> MRGSHHHHHHGSV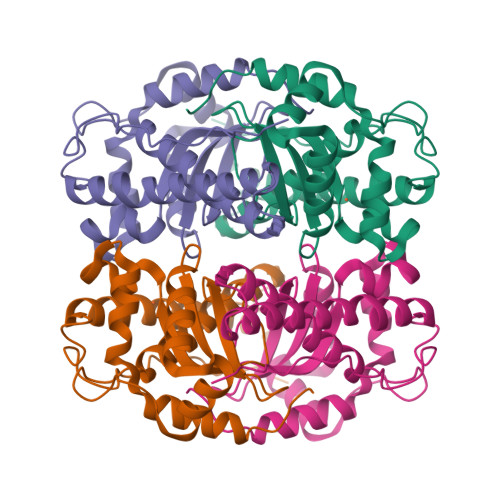VSLKRYELPPLPYNYDALEPIISAETLRYHHDKHHLGYVNGANAALDKLEKYLNGQLTDIDVRAVSRDFEFNYGGHILHTLYWLNMAPKGKGGGTPGGAIGDAINKFFGSFDKFKKLFGDAAKNVEGVGWAILAYDPVTGDLRILQVEKHNNVVTTNLIPLLAVDVFEHAYYIDYRNDRAKYVDSWWDLINWDDVEARYQKALNTPKLIL> MAATAAEAVASGSGEPREEAGALGPAWDESQLRSYSFPTRPIPRLSQSDPRAEELIENEEPVVLTDTNLVYPALKWDLEYLQENIGNGDFSVYSASTHKFLYYDEKKMANFQNFKPRSNREEMKFHEFVEKLQDIQQRGGEERLYLQQTLNDTVGRKIVMDFLGFNWNWINKQQGKRGWGQLTSNLLLIGMEGNVTPAHYDEQQNFFAQIKGYKRCILFPPDQFECLYPYPVHHPCDRQSQVDFDNPDYERFPNFQNVVGYETVVGPGDVLYIPMYWWHHIESLLNGGITITVNFWYKGAPTPKRIEYPLKAHQKVAIMRNIEKMLGEALGNPQEVGPLLNTMIKGRYN;> EVV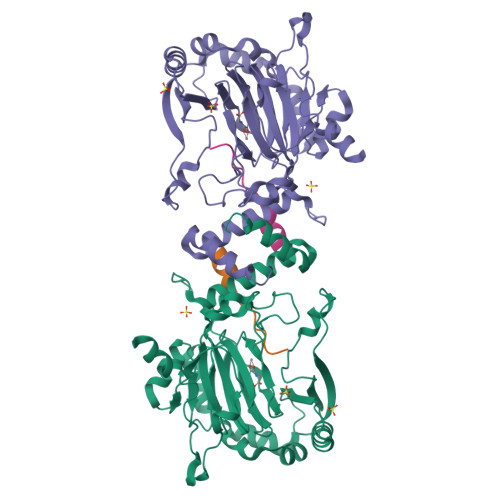KLLLEHGADVXA> MHHHHHHSSGRENLYFQGPEQPFIVLGQEEYGEHHSSIMHCRVDCSGRRVASLDVDGVIKVWSFNPIMQTKASSISKSPLLSLEWATKRDRLLLLGSGVGTVRLYDTEAKKNLCEININDNMPRILSLACSPNGASFVCSAAAPSLTSQVDFSAPDIGSKGMN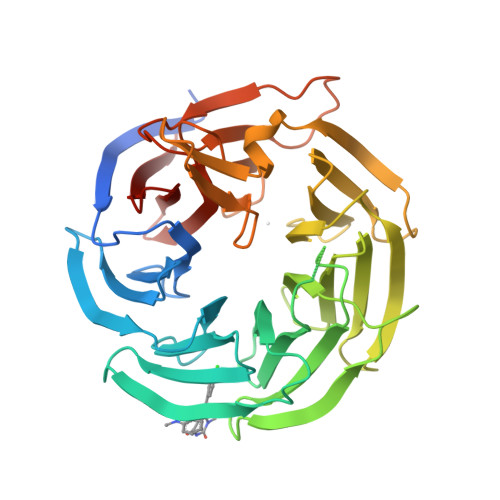QVPGRLLLWDTKTMKQQLQFSLDPEPIAINCTAFNHNGNLLVTGAADGVIRLFDMQQHECAMSWRAHYGEVYSVEFSYDENTVYSIGEDGKFIQWNIHKSGLKVSEYSLPSDATGPFVLSGYSGYKQVQVPRGRLFAFDSEGNYMLTCSATGGVIYKLGGDEKVLESCLSLGGHRAPVVTVDWSTAMDCGTCLTASMDGKIKLTTLLAHKA>GPGKRVYQIGSSSRD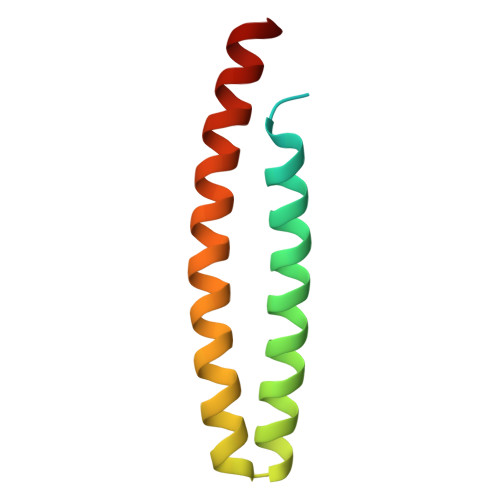VQVCPRGAGAALRQEIEDKQLMVNNLTDELQDAIDEANPAEIANTSQQLRHARADLADLQRRFAVLRNEDRRINQ[2x]Here, we report that c-di-GMP can assemble into a tetramer that mediates the effective dimerization of a transcription factor, BldD, which controls the progression of multicellular differentiation in sporulating actinomycete bacteria. BldD is an 18 kDa DNA-binding protein consisting of two distinct domains connected by a flexible linker. BldD sits at the top of the regulatory cascade controlling development, serving to repress expression of sporulation genes during vegetative growth (den Hengst et al., 2010). Specifically, structural and biochemical analyses show that the second messenger c-di-GMP activates BldD DNA binding by driving a unique form of dimerization that is mediated by a tetrameric form of c-di-GMP.

To elucidate the molecular basis for c-di-GMP recognition and binding by the BldD CTD and to gain insight into how this interaction may elicit developmental signaling, we determined structures of the S. venezuelae BldD CTD (residues 80–166) and S. coelicolor BldD CTD (residues 80–167) in complex with c-di-GMP. Three S. venezuelae BldD C-domain-(c-di-GMP) structures and one S. coelicolor BldD C-domain-(c-di-GMP) structure were determined to resolutions of 1.95 Å, 2.33 Å, 1.75 Å, and 2.25 Å, respectively (see Extended Experimental Procedures and Tables S1 and S2). The BldD CTD uses a previously unseen mode of c-di-GMP binding in which two noninteracting CTDs are glued together by a c-di-GMP tetramer composed of two interlocked c-di-GMP dimers. Indeed, the closest approach of any Cα atoms of the two tethered CTDs is ∼10 Å. The BldD CTD interacts with c-di-GMP using two contiguous surface motifs, herein called motif 1 and motif 2, which are located between the two β-α-α repeats. Motif 1 is composed of residues 114–116 (RGD) and motif 2 is composed of residues 125–128 (RQDD). Specifically, motif 2 from each CTD protomer combine to mediate contacts to one intercalated c-di-GMP dimer, Asp116 of motif 1 from each protomer combine to mediate contacts to the other c-di-GMP dimer, while Arg114 sits centrally and anchors both dimers. Arg114 is the only CTD residue that makes contacts to both intercalated c-di-GMP dimers. By sharp contrast, the BldD-bound tetrameric c-di-GMP is a tightly packed structure that is not secured by ions. Notably, the identical CTD dimer-(c-di-GMP) tetramer structure was seen in multiple crystal forms.

>GSHMEPPPKLVLDLERMAHVPQEKAGPLQRYAATIQSQRGDYNGKVLSIRQDDLRTLAVIYDQSPSVLTEQLISWGVLDADARRAVAHEEN[12x]> GEEERAFLVAREELASALRRDSGQAF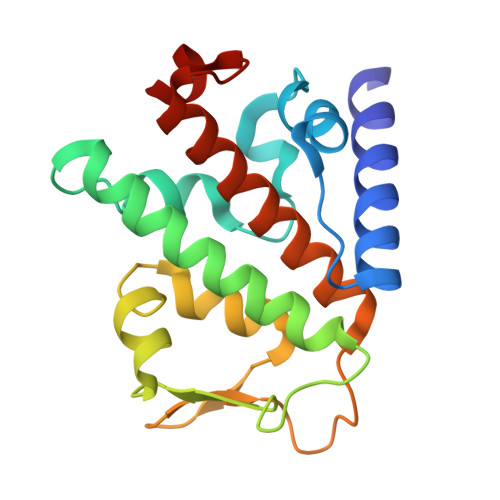SLEQLRPLLASSLPLAARYLQLDAARLVRCNAHGEPRNYLNTLSTALNILEKYGRNLLSPQRPRYWRGVKFNNPVFRSTVDAVQGGRDVLRLYGYTEEQPDGLSFPEGQEEPDEHQVATVTLEVLLLRTELSLLLQNTHPRQQALEQ>MQTKKNEIWVGIFLLAALLAALFVCLKAANVTSIRTEPTYTLYATFDNIGGLKARSPVSIGGVVVGRVADITLDPKTYLPRVTLEIEQRYNHIPDTSSLSIRTSGLLGEQYLALNVGFEDPELGTAILKDGDTIQDTKSAMVLEDLIGQFLYGSKGDDNKNSGDAPAAAPGNNETTEPVGTTK[6x];> MFKRLMMVALLVIAPLSAATAADQTNPYKLMDEAAQKTFDRLKNEQPQIRANPDYLRTIVDQELLPYVQVKYAGALVLGQYYKSATPAQREAYFAAFREYLKQAYGQALAMYHGQTYQIAPEQPLGDKTIVPIRVTIIDPNGRPPVRLD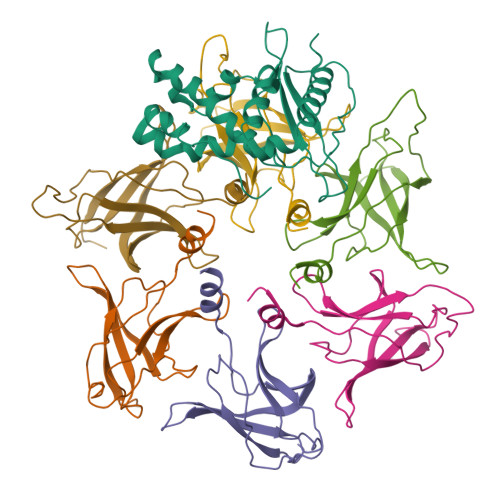FQWRKNSQTGNWQAYDMIAEGVSMITTKQNEWGTLLRTKGIDGLTAQLKSISQQKITLEEKK>[2x]MAE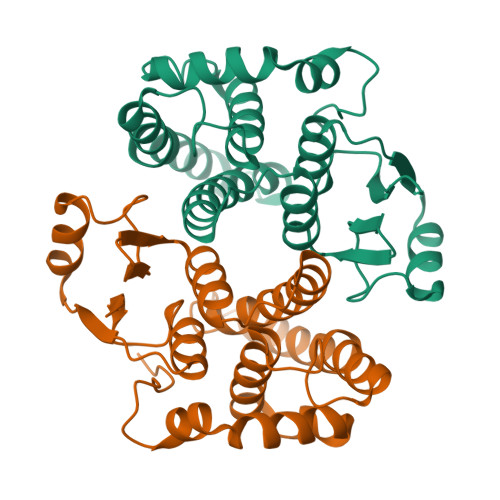KPKLHYFNARGRMESTRWLAAAAGVEFEEKFIKSAEDLDKLRNDGYLMFQQVPMVEIDGMKLVQTRAILNYIASKYNLYGKDIKERALIDMYIEGIADLGEMILLLPVCPPEEKDAKLALIKEKIKNRYFPAFEKVLKSHGQDYLVGNKLSRADIHLVELLYYVEELDSSLISSFPLLKALKTRISNLPTVKKFLQPGSPRKPPMDEKSLEEARKIFRF>MLPHGLIVSCQALPDEPLHSSFIMSKMALAAYEGGAVGIRANTKEDILAIKETVDLPVIGIVKRDYDHSDVFITATSKEVDELIESQCEVIALDATLQQRPKETLDELVSYIRTHAPNVEIMADIATVEEAK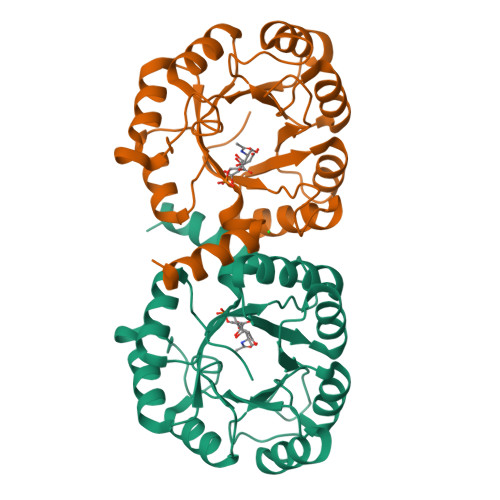NAARLGFDYIGTTLHGYTSYTQGQLLYQNDFQFLKDVLQSVDAKVIAEGNVITPDMYKRVMDLGVHCSVVGGAITRPKEITKRFVQIMED[2x]> MGVTCVSQMPVAEGKSVQQTVELLTRKLEMLGAEKQGTFCVDCETYHTAASTLGSQGQTGKLMYVMHNSEYPLSCFALFENGPCLIADTNFDVLMVKLKGFFQSAKASKIETRGTRYQYCDFLVKV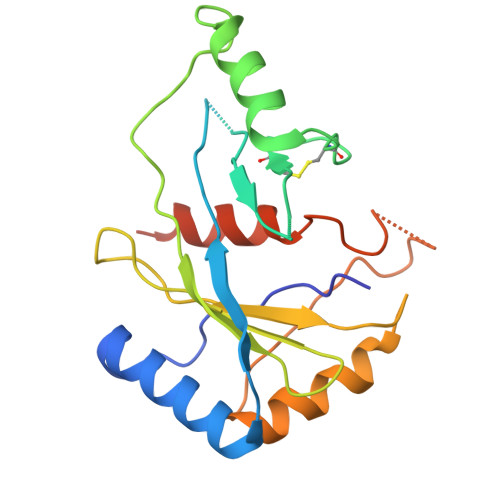GTVTMGPSARGISVEVEYGPCVVASDCWSLLLEFLQSFLGSHTPGAPAVFGNRHDAVYGPADTMVQYMELFNKIRKQQQVPVAGIR> QSDS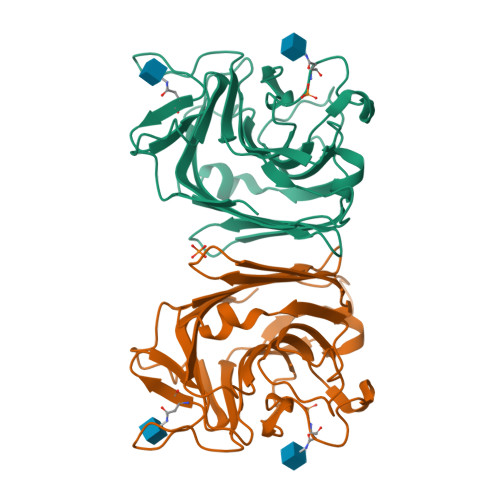VSFTFPNFWSDVEDSIIFQGDANTTAGTLQLCKTNQYGTPLQWSAGRALYSDPVQLWDNKTESVASFYTEFTFFLKITGNGPADGLAFFLAPPDSDVKDAGEYLGLFNKSTATQPSKNQVVAVEFDTWTNPNFPEPSYRHIGINVNSIVSVATKRWEDSDIFSGKIATARISYDGSAEILTVVLSYPDGSDYILSHSVDMRQNLPESVRVGISASTGNNQFLTVYILSWRFSSNLQSTSVKAAMEPEITRTVV DHDP reductase (DHDPR; dapB) is a branching enzyme associated with two described pathways and that reduces DHDP to tetrahydroDPA using NAD(P)H as a cofactor. DHDPR has two domains, including an N-terminal nucleotide-binding domain and a C-terminal domain for substrate binding and tetramerization. To address these issues, we determined the structure and characterized the biochemical properties of DHDPR from the psychrophilic bacterium Paenisporosarcina sp. TG-14 (PaDHDPR) isolated from sediment-laden, stratified basal ice from Taylor glacier, McMurdo dry valley, Antarctica29. The results of isothermal titration calorimetry (ITC) and enzyme activity assays demonstrated that PaDHDPR has a strong preference for NADPH as a cofactor.

The crystal structures of apo PaDHDPR (without the cofactor) and the DPA- and NADPH/DPA-bound forms of the enzyme were determined at 1.8 Å, 1.8 Å, and 2.1 Å resolutions, respectively. The final 1.8 Å high-resolution native model of PaDHDPR was refined and obtained by molecular replacement using the initial SAD-phasing model. PaDHDPR tetramerization was observed by analytical centrifugation and through generation of a crystallographic symmetry mate. The final model of the apo PaDHDPR monomer included 264 amino acid residues and 296 water molecules, with an overall topology comprising eight α-helices and 11 β-strands. DynDom analysis of PaDHDPR structures show distinct N- and C-terminal domains linked by two hinge regions (residues 129–133 and 233–235), with a 32.3° rotation angle and 2.1-Å translational movement. The N-terminal domain (residues 1–127 and 235–264) responsible for cofactor binding comprised a parallel six-stranded β-sheet surrounded by six α-helices. The C-terminal domain (residues 128–234) responsible for substrate binding and tetramer formation included a five-stranded β-sheet and two α-helices. In the tetramer, each C-terminal domain formed a central 20-stranded β-barrel structure surrounded by eight α-helices. In the apo form, this loop region shows a relatively high B-factor as compared with other regions. The apo and DPA-bound forms of PaDHDPR were in an open state, whereas the DPA/NADPH-bound enzyme was in a closed state.

> MIRVAIGGPRGKMGQEAVHTVMNNENMELVAVLDHKDIGDLLSESPNFPASYEVPVFLNLESLIVTIKPDVFLDLTTPHQVFEHTMLCLQNNVRPVIGTTGFTDEQLQQCTILAEVNKLGCIVAPNFAIGAVLMMKFASLAAAYFPDVEIIEMHHDQKLDAPSGTAYKTAQMIAEVRPSHKQGHPNEKETLEGARGASYDGIPIHSVRLPGLIAHQQILFGGEGQLFTLRHDSYNRQSFMSGVTFSINQVMEIKELVYGLENIL The recombination mediator complex RecFOR, consisting of the RecF, RecO, and RecR proteins, is needed to initiate homologous recombination in bacteria by positioning the recombinase protein RecA on damaged DNA. Bacteria from the phylum Campylobacterota, such as the pathogen Campylobacter jejuni, lack the recF gene and trigger homologous recombination using only RecR and RecO. Given that RecR interacts with RecF or RecO for the initiation of homologous recombination, RecR functions as the most critical recombination mediator protein in both the RecFOR and RecOR pathways. To elucidate the functional properties of C. jejuni RecR (cjRecR) in recombination initiation that differ from or are similar to those in RecF-expressing bacteria, we determined the crystal structure of cjRecR and performed structure-based binding analyses. cjRecR forms a rectangular ring-like tetrameric structure and coordinates a zinc ion using four cysteine residues, as observed for RecR proteins from RecF-expressing bacteria.

The crystal structure of cjRecR was obtained at a 2.6 Å resolution using the recombinantly expressed cjRecR protein (residues 1–190). The structure of a cjRecR monomer (residues 1–189) consists of seven α-helices (α1–α7) and six β-strands (β1–β6) and is spatially separated into three parts, including the N-terminal domain (NTD), middle domain (MD), and C-terminal domain (CTD). The four cjRecR chains from the asymmetric unit assemble into a tetramer in the shape of a rectangular ring with a central pore, as observed for other RecR structures. cjRecR tetramerization is mainly mediated by NTD-NTD′ homodimerization and MD-CTD′ heterodimerization (the prime denotes another polypeptide chain). The zinc ion is simultaneously coordinated by four conserved cysteine residues (C58, C61, C70, and C73) from the two CxxC motifs at the β1–β2 and β2–β3 loops, stabilizing the relatively long β1–β2 and β2–β3 loops, which would otherwise be highly flexible. Therefore, we conclude that zinc ion coordination by the cysteine residues is required to maintain the protein stability of cjRecR. The positive patch of cjRecR in the central pore includes positively charged residues, K23, K24, R28, and K90, from each cjRecR chain. In contrast to the cjRecR K24 and R28 residues, cjRecR K23 and K90 are conserved as positively charged residues in the phylum Campylobacterota and are generally replaced with neutral residues in other bacterial phyla, most species of which, including C. subterraneus and D. radiodurans, have the recF gene, highlighting the unique role of the additional positive residues in DNA recognition by Campylobacterota RecR proteins. First, cjRecR substantially interacted with ssDNA, with a Kd value of 6.8 μM, in contrast to drRecR and csRecR. cjRecR exhibits the largest structural difference in the β4–α5 loop of the Toprim subdomain from the structurally defined RecR orthologs from RecF-expressing bacteria, including ttRecR, csRecR, paRecR, and drRecR.

>[4x]GSAKDPMVKGLEKFNELVESFANLPTIGKKTAIRLAYHLCINNQIDGMKLAHNIENAIRFIKPCEQCGALSENELCEICSDKERNKNILCIVESPKDILTLEESQSYNGLYFVLDELNEEKLEKLKQIILKLNISELIFALTHSINSDATIFFIEDKFKGLNLTFSKIAQGIPSGVNLENVDLISLNKAMNFRTKI> TVLPKDIPGDSLKVTVGTANGKPGDTVTVPVTFADVAKMKNVGTCNFYLGYDASLLEVVSVDAGPIVKNAAVNFSSSASNGTISFLFLDNTITDELITADGVFANIKFKLKSVTAKTTTPVTFKDGGAFGDGTMSKIASVTK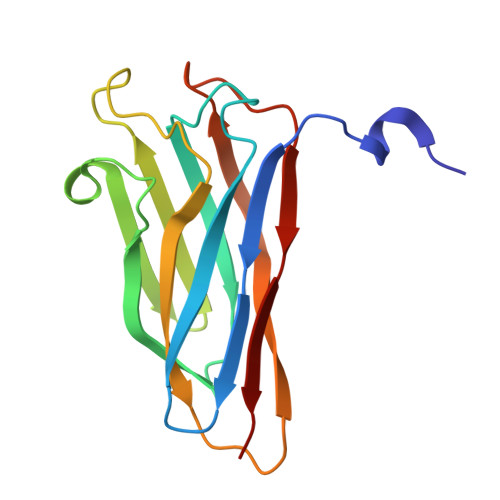TNGSVTIDP> MRGSHHHHHHGSAEKQERVQHLHDIRDLHRYYSSESFEYSNVSGKVENYNGSNVVRFNPQNHQLFLLGKDKEQYKEGLQGQNVFVVQELIDPNGRLSTVGGVTKKNNKTSETNTPLFVNKVNGEDLDASIDSFLIQKEEISLKELDFKIRQQLVNN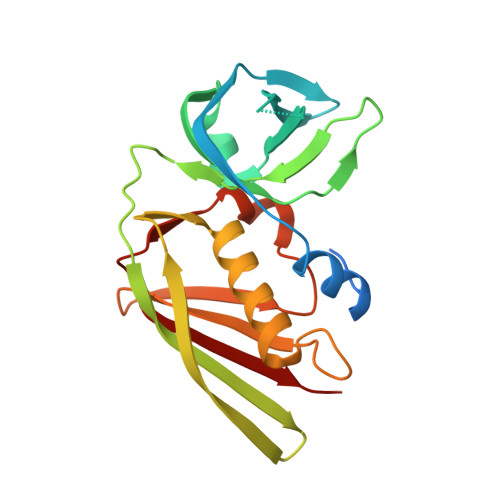YGLYKGTSKYGKIIINLKDENKVEIDLGDKLQFERMGDVLNSKDIRGISVTINQI> GSPEFPGRLSRTSVQTEDDQLIAGQSARAIMAQLPQEEKAKIAEQVEIFHQEKSKLDAEVAKWDDSGNDIIVLAKQMCMIMMEMTDFTRGKGPLKNTSDVINAAKKIAEAGSRMDKLARAVADQCPDSACKQDLLAYLQRIALYCHQLNICSKVKAEVQNLGGELIVSGLDSATSLIQAAKNLMN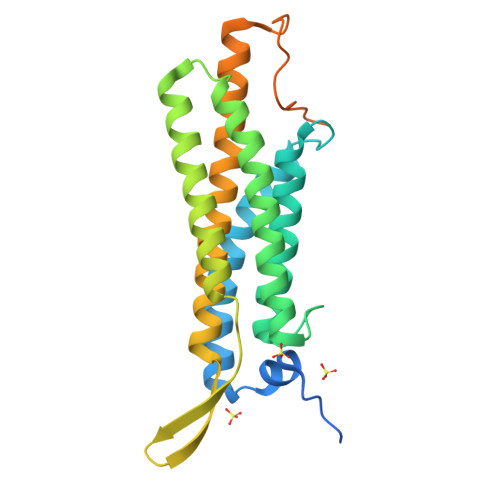AVVLTVKASYVASTKYQKVYGTAAVNSPVVSWKMKAPEKKPLVKREKPEEFQTRVRRGSQKKHISPVQALSEFKAMDSF>MNRGVIVTGGGHGIGKQICLDFLEAGDKVCFIDIDEKRSADFAKERPNLFYFHGDVADPLTLKKFVEYAMEKLQRIDVLVNNACRGSKGILSSLLYEEFDYILSVGLKAPYELSRLCRDELIKNKGRIINIASTRAFQSEPDSEAYASAKGGIVALTHALAMSLGPDVLVNCIAPGWINVTEQQEFTQEDCAAIPAGKVGTPKDISNMVLFLCQQDFITGETIIVDGGMSKRMIYHGDWN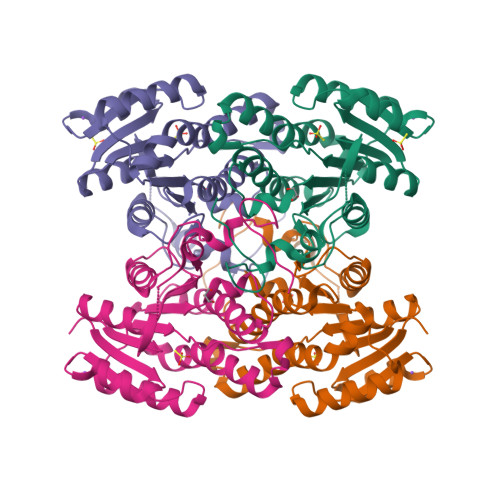WFYKIDK[2x]N-[(1S)-1-{[(1S)-5-AMINO-1-[(2-CYCLOHEXYLETHYL)CARBAMOYL]PENTYL]CARBAMOYL}-2-HYDROXYETHYL]-10-HYDROXYDECANAMIDE 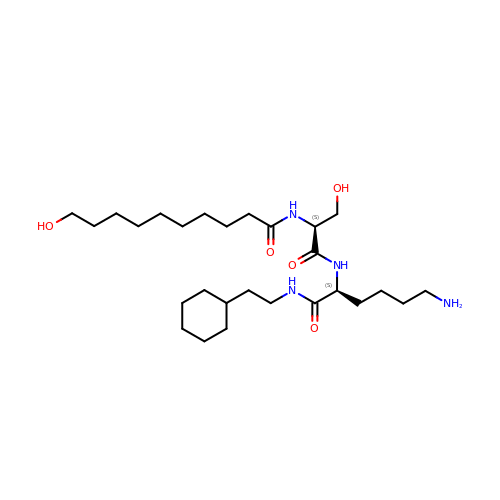| C27 H52 N4 O5 | WOFDCVFMMXKBIZ-ZEQRLZLVSA-N> MYVCHFENCGKAFKKHNQLKVHQFSHTQQLPYECPHEGCDKRFSLPSRLKRHEKV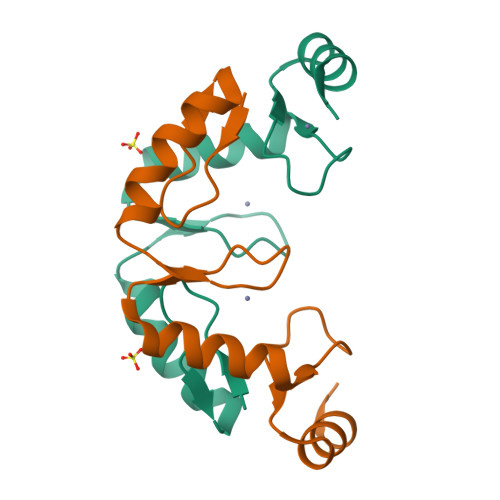HAGYPCKKDDSCSFVGKTWTLYLKHVAECH> MQIITAEDYRLYGGLKRPELESGVEVMITAANALITSLLGMDDADAVDQLITTKPTRKKYFLSSPSATSVTKMTINDKEIDPEQYKL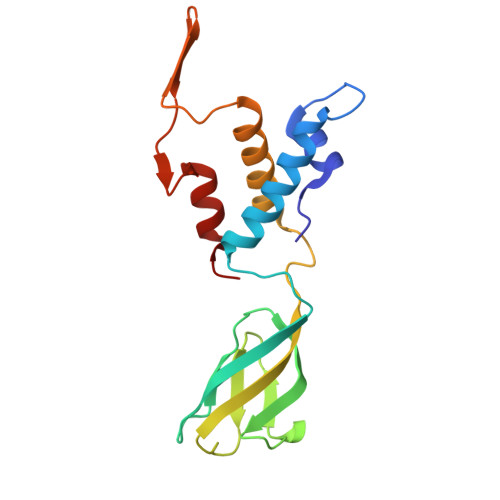YSDGVILLKFNPPEGYMDVEYTQGGFNPMPEDLKLAACMLVDHWHKQDYRQARTIGGETVTFNNTKSGIPEHIRTIIEVYRRV> GLPVLNTPGSNQYLTSDNHQSPCAIPEFDVTPPIDIPGEVKNMMELAEIDTMIPLNLESTKRNTMDMYRVTLSDSADLSQPILCLSLSPAFDPRLSHTMLGEVLNYYTHWAGSLKFTFLFCGSMMATGKILVA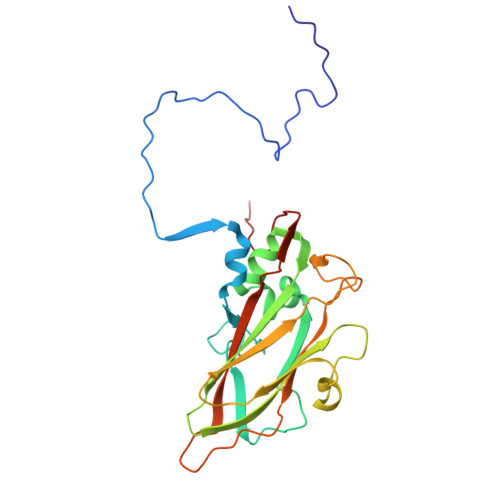YAPPGAQPPTSRKEAMLGTHVIWDLGLQSSCTMVVPWISNVTYRQTTQDSFTEGGYISMFYQTRIVVPLSTPKSMSMLGFVSACNDFSVRLLRDTTHISQSALPQ> MSEKKVHLRLRKELSVPIAVVENESLAQLSYEEESQASLMDISMEQQQLRLHSHFDNSKVFTENNRYIVKTLQTDYSSGFSNDDELNGYIDMQIGYGLVNDHKKVYIWNIHSTQKDTPYITVPFRSDDNDEIAVAPRCILTFPATMDESPLALNPNDQDETGGLIIIKGSKAIYYEDINSINNLNFKLSEKFSHELELPINSSGGEKCDLMLNCEPAGIVLSTNMGRIFFITIRNSMGKPQLKLGKLLNKPFKLGIWSKIFNTNSSVVSLRNGPILGKGTRLVYITTNKGIFQTWQLSATNSHPTKLIDVNIYEAILESLQDLYPFAHGTLKIWDSHPLQDESSQLFLSSIYDSSCNETYYILSTIIFDSSSNSFTIFSTYRLNTFMESITDTKFKPKIFIPQMENANDTNEVTSILVMFPNAVVITQVNSKLDSSYSMRRKWEDIVSLRNDIDIIGSGYDSKSLYVLTKQMGVLQFFVKENEETNSKPEVGFVKSHVDQAVYFSKINANPIDFNLPPEISLDQESIEHDLKLTSEEIFHSNGKYIPPMLNTLGQHLSVRKEFFQNFLTFVAKNFNYKISPELKLDLIEKFEILNCCIKFNSIIRQSDVLNDIWEKTLSNYNLTQNEHLTTKTVVINSPDVFPVIFKQFLNHVVFVLFPSQNQNFKLNVTNLINLCFYDGILEEGEKTIRYELLELDPMEVDTSKLPWFINFDYLNCINQCFFDFTFACEEEGSLDSYKEGLLKIVKILYYQFNQFKIWINTQPVKSVNANDNFININNLYDDNHLDWNHVLCKVNLKEQCIQIAEFYKDLSGLVQTLQTLDQNDSTTVSLYETFFNEFPKEFSFTLFEYLIKHKKLNDLIFRFPQQHDVLIQFFQESAPKYGHVAWIQQILDGSYADAMNTLKNITVDDSKKGESLSECELHLNVAKLSSLLVEKDNLDINTLRKIQYNLDTIDAEKNISNKLKKGEVQICKRFKNGSIREVFNILVEELKSTTVVNLSDLVELYSMLDDEESLFIPLRLLSVDGNLLNFEVKKFLNALVWRRIVLLNASNEGDKLLQHIVKRVFDEELPKNNDFPLPSVDLLCDKSLLTPEYISETYGRFPIDQNAIREEIYEEISQVETLNSDNSLEIKLHSTIGSVAKEKNYTINY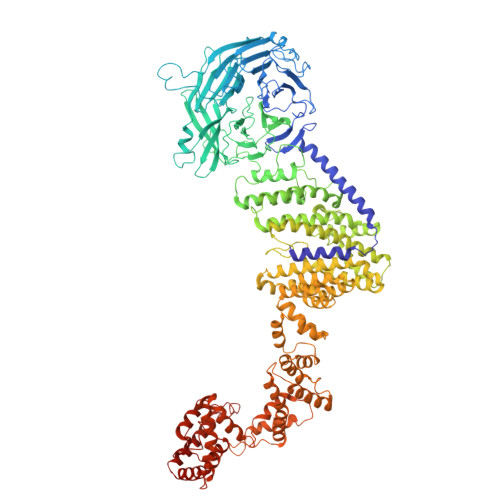ETNTVEY> DDPVKVRKWKHVQM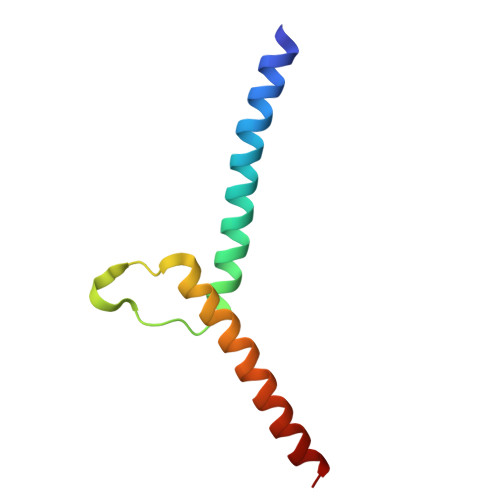EKIRRINTKEAFERLIKSVRTPPKENGKRIPKHILLTCVMNDIKSIRSANEALQHILDD The packaging of cargo transmembrane proteins into COPII-coated vesicles entails a direct interaction between COPII protein and cytoplasmically-oriented ER export signals. About a half dozen export signals have been identified to date, almost all comprising short peptide motifs, all of them binding to the Sec24 subunit of the COPII inner coat. The ΦC export signal was identified in studies of p24-family and ERGIC-53 proteins, and comprises a C-terminal signature of a pair of hydrophobic residues or a single terminal valine residue. The ΦC motif contacts a site on Sec24a that is also the binding site for the LxxLE- and DxE-class export motifs (Miller et al., 2003; Mossessova et al., 2003).

A series of ΦC-signal peptides was synthesized, based on a core sequence of yeast Emp24p, and individual peptides were soaked at high concentrations into two crystal forms of human COPII protein: one comprising Sec23a/Sec24a•Sec22b, the other Sec24c. For all ΦC sequences, we observed clear evidence for peptide binding to a site on Sec24a in the Sec23a/Sec24a•Sec22b crystals, based on the presence of residual electron density that matches the peptide sequence (this binding site is occluded in the Sec24c crystals). (D) Schematic diagram shows the bonding arrangement to the potent ΦC motif Leu-Val. Diagram is based on the structure of Sec23a/Sec24a•Sec22b bound to the sequence EVTSLV. The label N denotes the serine residue upstream of the Leu-Val motif. Thus, specific recognition of the ΦC motif involves the terminal carboxylate group bonding to Arg750 and Arg752 of Sec24a, with the penultimate hydrophobic residue of the motif nestling against Tyr496, and the terminal hydrophobic residue fitting to a pocket of hydrophobic side chains.

> MTTYLEFIQQNEERDGVRFSWNVWPSSRLEATRMVVPVAALFTPLKERPDLPPIQYEPVLCSRTTCRAVLNPLCQVDYRAKLWACNFCYQRNQFPPSYAGISELNQPAELLPQFSSIEYVVLRGPQMPLIFLYVVDTCMEDEDLQALKESMQMSLSLLPPTALVGLITFGRMVQVHELGCEGISKSYVFRGTKDLSAKQLQEMLGLSKVPLTQATRGPQVQQPPPSNRFLQPVQKIDMNLTDLLGELQRDPWPVPQGKRPLRSSGVALSIAVGLLECTFPNTGARIMMFIGGPATQGPGMVVGDELKTPIRSWHDIDKDNAKYVKKGTKHFEALANRAATTGHVIDIYACALDQTGLLEMKCCPNLTGGYMVMGDSFNTSLFKQTFQRVFTKDMHGQFKMGFGGTLEIKTSREIKISGAIGPCVSLNSKGPCVSENEIGTGGTCQWKICGLSPTTTLAIYFEVVNQHNAPIPQGGRGAIQFVTQYQHSSGQRRIRVTTIARNWADAQTQIQNIAASFDQEAAAILMARLAIYRAETEEGPDVLRWLDRQLIRLCQKFGEYHKDDPSSFRFSETFSLYPQFMFHLRRSSFLQVFNNSPDESSYYRHHFMRQDLTQSLIMIQPILYAYSFSGPPEPVLLDSSSILADRILLMDTFFQILIYHGETIAQWRKSGYQDMPEYENFRHLLQAPVDDAQEILHSRFPMPRYIDTEHGGSQARFLLSKVNPSQTHNNMYAWGQESGAPILTDDVSLQVFMDHLKKLAVSSA;> EGLRVVNLLQERNMLPSTPLKPPVPNLHEDIQKLNCNPELFRCTLTSIPQTQALLNKAKLPLGLLLHPFKDLVQLPVVTSSTIVRCRSCRTYINPFVSFLDQRRWKCNLCYRVNDVPEEFLYNPLTRVYGEPHRRPEVQNATIEFMAPSEYMLRPPQPPVYLFVFDVSHNAVETGYLNSVCQSLLDNLDLLPGNTRTKIGFITFDSTIHFYGLQESLSQPQMLIVSDIEDVFIPMPENLLVNLNESKELVQDLLKTLPQMFTKTLETQSALGPALQAAFKLMSPTGGRMSVFQTQLPTLGVGALKPREEPNHRSSAKDIHMTPSTDFYKKLALDCSGQQVAVDLFLLSGQYSDLASLGCISRYSAGSVYYYPSYHHQHNPVQVQKLQKELQRYLTRKIGFEAVMRIRCTKGLSIHTFHGNFFVRSTDLLSLPNVNPDAGYAVQMSVEESLTDTQLVSFQSALLYTSSKGERRIRVHTLCLPVVSTLNDVFLGADVQAISGLLANMAVDRSMTASLSDARDALVNAVIDSLSAYRSSVLSNQQPGLMVPFSLRLFPLFVLALLKQKSFQTGTNARLDERIFAMCQVKNQPLVYLMLTTHPSLYRVDNLSDEGALNISDRTIPQPPILQLSVEKLSRDGAFLMDAGSVLMLWVGKNCTQNFLSQVLGVQNYASIPQPMTDLPELDTPESARIIAFISWLREQRPFFPILYVIADESPMKANFLQNMIEDRTESALSYYEFLLHIQQQVNK;> MVLLTMIARVADGLPLAASMQEDEQSGRDLQQYQSQAKQLFRKLNEQSPTRCTLEAGAMTFHYIIEQGVCYLVLCEAAFPKKLAFAYLEDLHSEFDEQHGKKVPTVSRPYSFIEFDTFIQKTKKLYIDSRARRNLGSINTELQDVQRIMVANIEEVL;> SLV>MSKTTPTKDSIRAEFEELVEKDSFWSKFVGSQFVSMLTLFITQIVYRCFQYADAALAEGFISTATRRSSILAAAETNSYVGTKPTPSSGMIEITATSEDAPAVIPKNMPLISDDQYPYMTMDVCRLVDGTGTVEVAQLEIQEVTYTVTAAKEFLEVVLSKALTAVCYKLEVFVTTDGKTTQWSSSTMFRLAGSKSQVYVEFYKPSEQLGVRFGDGLIGQIPPEGSTITLKVWCTNGDITLVAGQNLTPVDSAANLANLISVKTTTPITAGTDAETTEITRNRAQYYLAYDDQVVWGGDYTYFLVRNIPGLSWVKAWGEGQQEKLDGAYNVQNINKIFISGWHPNKSQSELEEMILAAFKKVPNELNKKFSYKEVRKLPFKITITGRISASLTIENVTDELKSALETKFGRDSTFFDPNRVGKYILIKKKDVWAFIETLGYFRDFYLEFVEWNESNGFYDFVYLDTENSTFNISYEEE[12x];>[6x]MGLNVASVKSYVSSALTTTLFGSGVGEREVGKLTSIIMNKMLFAQGWQFSVEVDGLEGADFFAKDITYHDYSIEYETIKIGGGNILQPTERSPGQITMMVRDTVDGLVLDWFKTAKSRVINPDGTGNIPSQYLLNVRIYRLLSSGLTKLENEMTVFPVTTGDVTYARDQVTEFKSFPMTFALHSTFNQSSSSLASLLGFSFSL;>MSQYSIQQSLGNASGVAVSPINADATLSTGVALNSSLWAGIGVFARGKPFTVLAVTESNYEDVLGEPLKPSSGSQFEPIRHVYEAIQQTSGYVVRAVPDDAKFPIIMFDESGEPAYSALPYGSEIELDSGEAFAIYVDDGDPCISPTRELTIETATADSAGNERFLLKLTQTTSLGVVTTLETHTVSLAEEAKDDMGRLCYLPTALEARSKYLRAVVNEELISTAKVTNKKSLAFTGGTNGDQSKISTAAYLRAVKVLNNAPYMYTAVLGLGCYDNAAITALGKICADRLIDGFFDVKPTLTYAEALPAVEDTGLLGTDYVSCSVYHYPFSCKDKWTQSRVVFGLSGVAYAAKARGVKKNSDVGGWHYSPAGEERAVIARASIQPLYPEDTPDEEAMVKGRLNKVSVGTSGQMIIDDALTCCTQDNYLHFQHVPSLMNAISRFFVQLARQMKHSPDGITAAGLTKGMTKLLDRFVASGALVAPRDPDADGTEPYVLKVTQAEFDKWEVVWACCPTGVARRIQGVPLLIK[30x];>[18x]MGHNNTKGNRKFIKGRYTANAAKGER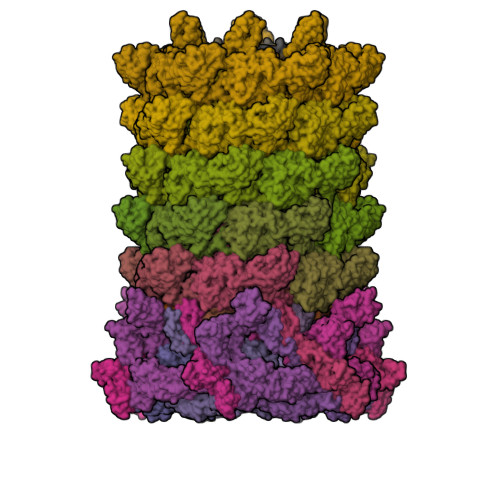LVSSEFLLTFAGHEDISVLVRTSQIPEMTREDVEDYGPNGVKFNQHGPIRNSGEIQVQCVETIEGDILQFIKDRIAAKDYVDITMAATPESKSSGVNAVTKAATTIEMLDCKIYSDAIDFSTEDVTAAVRPSLRIVYNWIEWD;>[6x]MAPIAYGVYSQADGVSPYLKVTLTNSQYQVTGYISQGAAMNMAQNWEAPFTGMSMGSVSGALGGFVQVGTETTSVARWNSLMVWEGGTPPTFTLPVTFIALNNPFIEVSGAIAALTAMISPELKAANVGGQIPERVTLNIGRRINITDVAIQDLSFDLDAPRDSNGYFLKNTVNLQLTGSSIYNSSDIVRAFQ;>[6x]MANNNEIDPLLTLELSGVKTYESQEEAWGARLYEWLNTYQGEVYGDPSWGNVLPQFKHEPTNLSHVQIAVEAMLLQKLTVDLPDIPISGLSVAEGDAFDKLKISIRIRDITITQDVVL;>[6x]MATSITTTQSTRQYPLSRYDDRNIADPILRAELRKEVMLMCESNDKNLTIYYVLPDEQYRPDLLAYRMWGIAELRWVVTLAAGLEDESQGMTVGKKLKLPPATWIREMIRHFQYDGQVIGTLSIA;>[6x]MQRSWFNHRLTSAKQKSLLYKSLADLVQSMMDTFVDPWLERITNRKSIFSMSKEDLETRTNELGQFFTIRTSNSSSVPMLLQQRLDEIHFKGTERPINQTIYREFNGISVLWDPIYAPVDLERHPYGTVLIPESTLETTGGTFGEMFLTSRGMISIPINDLARTMGITGTIDQSAITEEILRKFNQFVKPLLPLHIVFDGLTLYLSVVVNEHADMITLNEISDTEKAYCWFETSDTTSLTGVTSISAPITATPGGTIVKATPTFDRTRADDLLLDSDA>SNADSLPERIDLFVSLFDYNSATTSYDIRSIQTDFPTRLLTPDSMLPQTSEYPLKDIQLLYKLAQSCTGKLPLSPLITEPLVFTRSLCKGSSLSPRWFARSGLIHPGGGTYAFRYAEKYPAQFANLLPYMHIQERPNAAEGTLLYHLQNMGEDAINALVSGASMFGSGSDLWLRKGDIYYLFNEETWLTN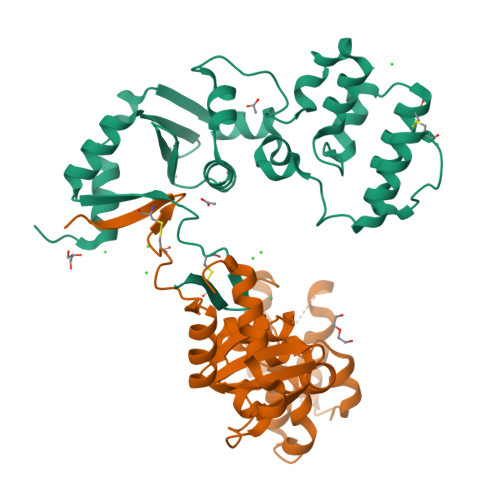ANKAGLSYSLLSADNTCFIQRGNICWDVEDHS[4x]PYRUVIC ACID | C3 H4 O3 | 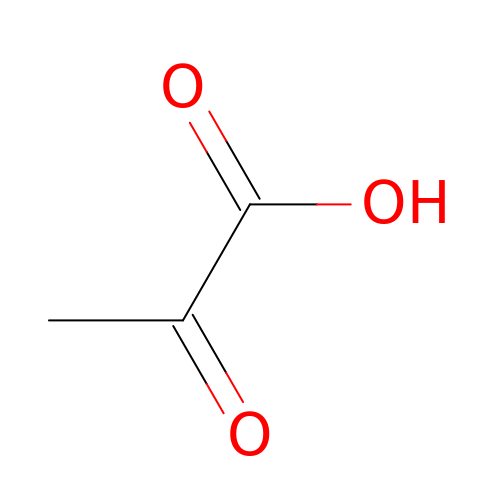LCTONWCANYUPML-UHFFFAOYSA-N> QSEPWTVLAHKKPQKDWKAYNPKTMRPPPLPEGTKCVKVMTWNVNGLRGLLKFESFSALQLAQRENFDILC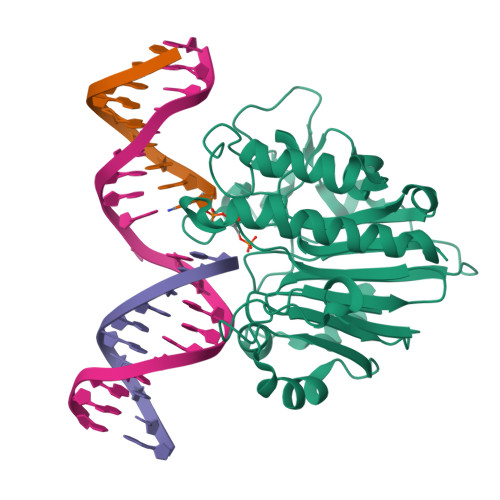LQETKLQVKDVEEIKKTLIDGYDHSFWSCSVSKLGYSGTAIISRIKPLSVRYGTGLSGHDTEGRIVTAEFDSFYLINTYVPNSGDGLKRLSYRIEEWDRTLSNHIKELEKSKPVVLTGDLNCAHEEIDIFNPAGNKRSAGFTIEERQSFGANLLDKGFVDTFRKQHPGVVGYTYWGYRHGGRKTNKGWRLDYFLVSQSIAANVHDSYILPDINGSDHCPIGLILKL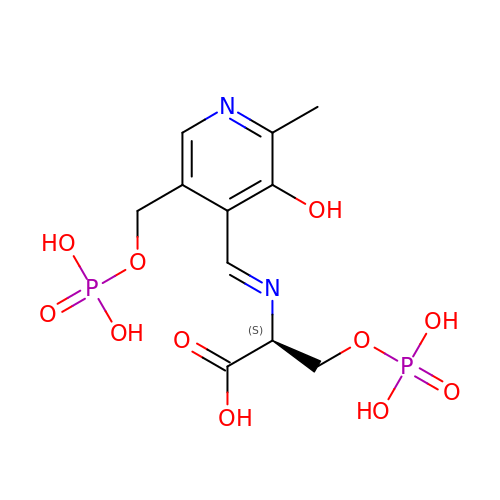(2S)-2-[(E)-[2-methyl-3-oxidanyl-5-(phosphonooxymethyl)pyridin-4-yl]methylideneamino]-3-phosphonooxy-propanoic acid | C11 H16 N2 O11 P2 | OWXVBOWGCHCIMU-VIFPVBQESA-N> GKKAGNNTLRPVTIRQILNAEQPHPDAEFILDGAELGQLTFVAVVRNISRNATNVAYSVEDGTGQIEVRQWLDSSSDDSSKASEIRNNVYVRVLGTLK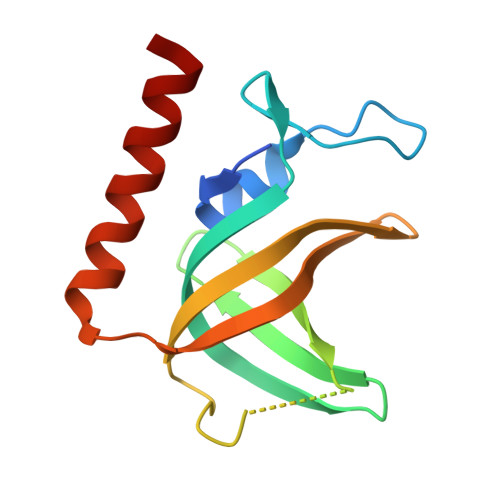SFQNRRSISSGHMRPVIDYNEVMFHRLEAVHAHLQVTR> TGRA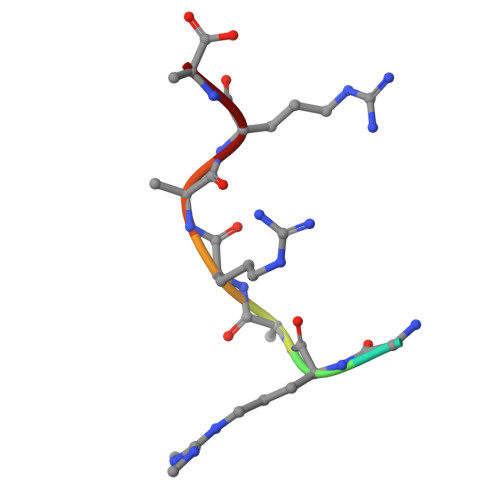RARA>[2x]MIKSKGDVNILLNFRHNINGEDLIIAVAQDHETGEVLMVAYMNREALRRTLETGTAHYWSTS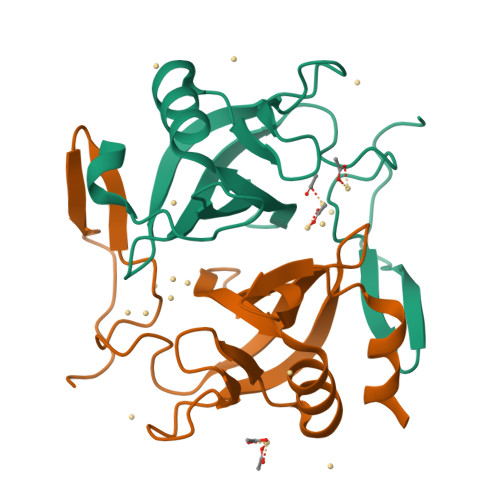RGKLWLKGESSGHVQRVKDVLVDCDGDAVVLKVEQEGGACHTGYRSCFYRSIDGDELKVREDAVKVFDPEEIYGDG>MTIHPTAIID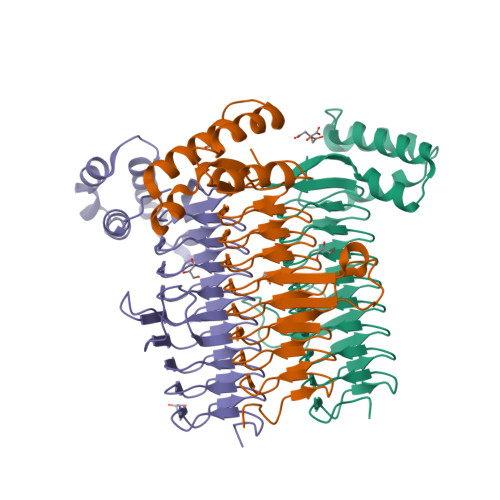KSAMIADSAIIGPYCIVGKNSQIGAHTVLRSHVIIGENTKIGVHNDIYQFASIGENPQDLKYAGEQTYLEIGDHNRIREACTIHRGTVQDRGITRIGNQNLLMVNVHIAHDCVVGDDNVLANNVGVAGHAHIGNHVIIGGQSGVHQFCRIDDYSMVGGASLIVKDVAAYVMASGNPAKAHGLNKEGMRRKGWSKDTIKALDEAYRLVFRSGLLRDEALDELTKLVEKEPKIQLLIDSINNSKRGLVR[6x]> DEKRLHFGNGHLKLPGLRTYVDPHTYEDPTQTVHEFAKELDATNISIDKVVGAGEFGEV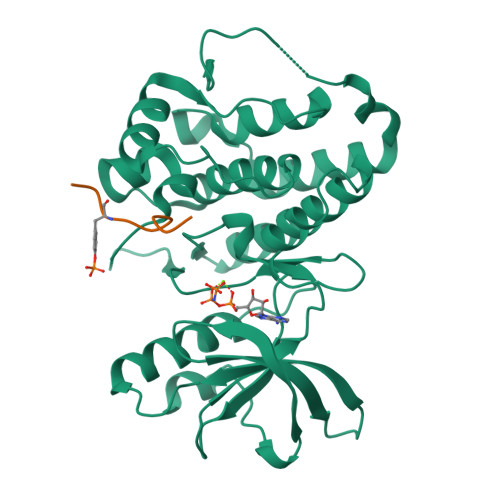CSGRLKLPSKKEISVAIKTLKVGYTEKQRRDFLGEASIMGQFDHPNIIRLEGVVTKSKPVMIVTEYMENGSLDSFLRKHDAQFTVIQLVGMLRGIASGMKYLSDMGYVHRDLAARNILINSNLVCKVSDFGLSRVLEDDPEAAYTTRGGKIPIRWTSPEAIAYRKFTSASDVWSYGIVLWEVMSYGERPYWEMSNQDVIKAVDEGYRLPPPMDCPAALYQLMLDCWQKDRNNRPKFEQIVSILDKLIRNPGSLKIITSAAARPSNLLLDQSNVDITTFRTTGDWLNGVWTAHCKEIFTGVEYSSCDTIAKIS;> KQWDNYEYIW N-[(2S)-3-(9H-carbazol-9-yl)-2-hydroxypropyl]-N-(furan-2-ylmethyl)methanesulfonamide | C21 H22 N2 O4 S | 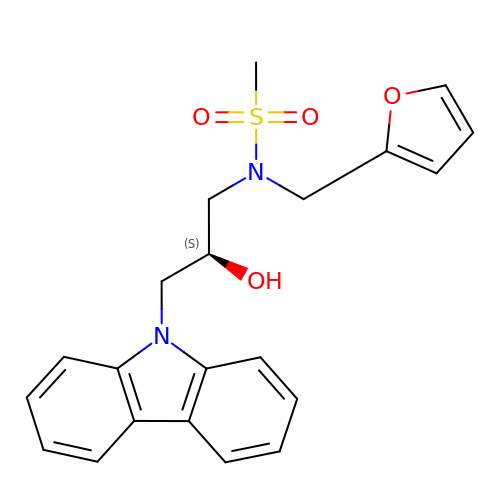OQAFDLPAPSSOHY-MRXNPFEDSA-N> MG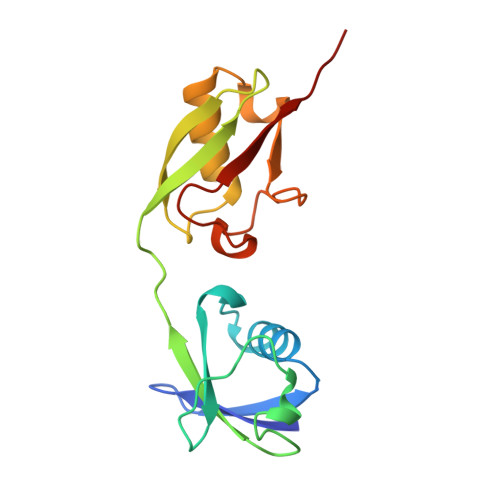WDLTVKMLAGNEFQVSLSSSMSVSELKAQITQKIGVHAFQQRLAVHPSGVALQDRVPLASQGLGPGSTVLLVVDKSDEPLNILVRNNKGRSSTYEVRLTQTVAHLKQQVSGLEGVQDDLFWLTFEGKPLEDQLPLGEYGLKPLSTVFMNLRLRG> XAACLRR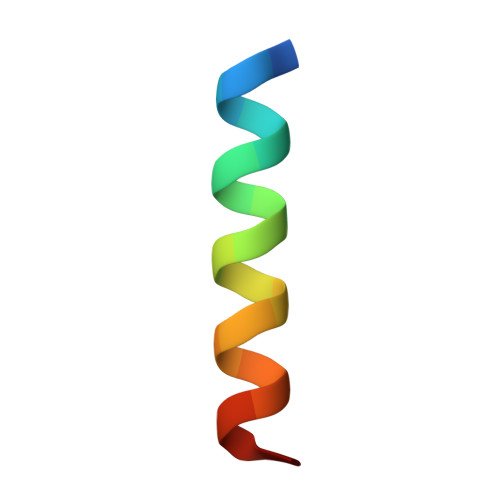IGDCVNLRQKLLNX> MDYKDDDDKSQKNGIATLLQAEKEAHEIVSKARKYRQDKLKQAKTDAAKEIDSYKIQKDKELKEFEQKNAGGVGELEKKAEA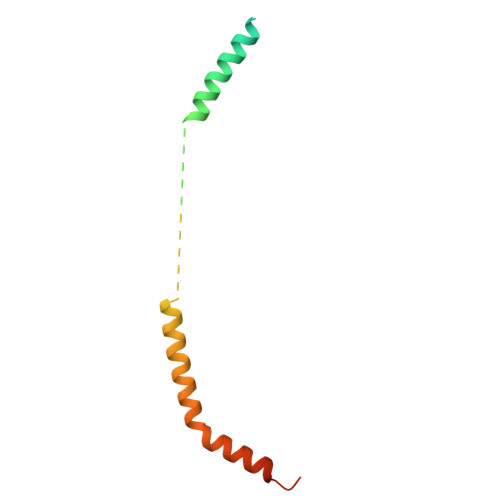GVQGELAEIKKIAEKKKDDVVKILIETVIKPSAEVHINAL3'-OXO-ADENOSINE | C10 H11 N5 O4 | 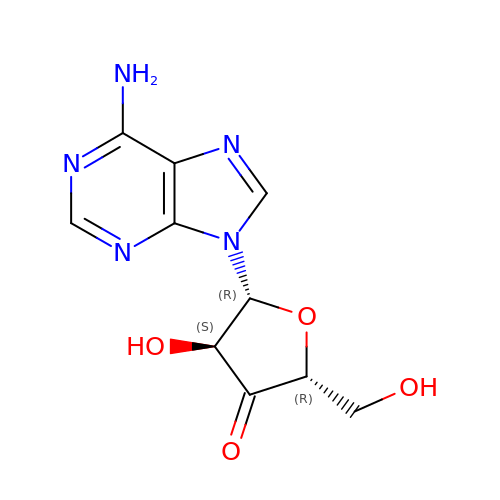MIAZJCOESMXYNJ-XMRAEQSQSA-N> TGKELLLVLYDYQEKSPREITVKKGDILTLLNSTNKDWWKVEF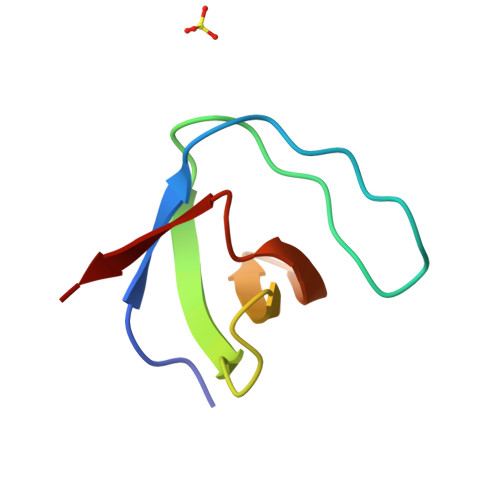NDRQGFLPAAYLKKLD> SPFSIFHPNIQAAKDCNQVRDFITKEVDSDVNTA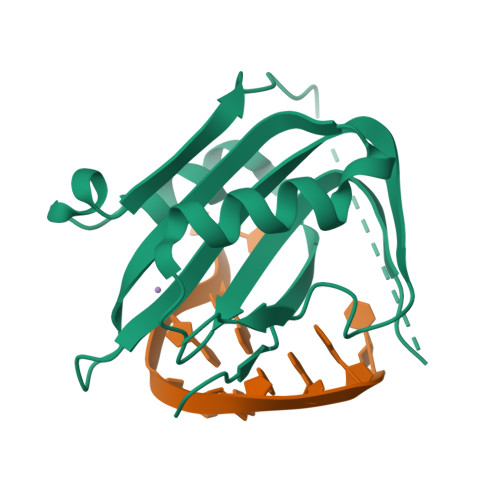EWGTFVAVSTPGRKDRDADMASSSTPRFRVYSKYLFLTYPQCTLEPQYALDSLRTLLNKYEPLYIAAVRELHEDGSPHLHVLVQNKLRASITNPNALNLRMDT> MGESQTLDKVYQMKSKPRGYCLIINNHNF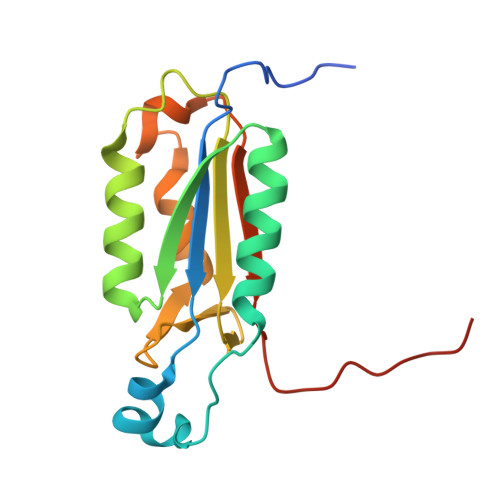AKAREKVPKLHSIRDRNGTHLDAGALTTTFEELHFEIKPHDDCTVEQIYEILKIYQLMDHSNMDCFICCILSHGDKGIIYGTDGQEAPIYELTSQFTGLKCPSLAGKPKVFFIQACQGDNYQKGIPVETD2-(2-methoxyphenyl)-6-[[4-(4-methylpiperazin-1-yl)phenyl]amino]-1-[6-(2-oxidanylpropan-2-yl)pyridin-2-yl]pyrazolo[3,4-d]pyrimidin-3-one 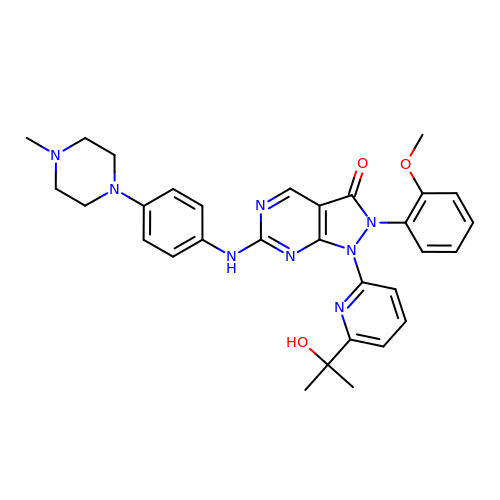| C31 H34 N8 O3 | YRSUINBEIRGTSA-UHFFFAOYSA-N> MPKALIVYGSTTGNTEYTAETIARQLANAGYEVD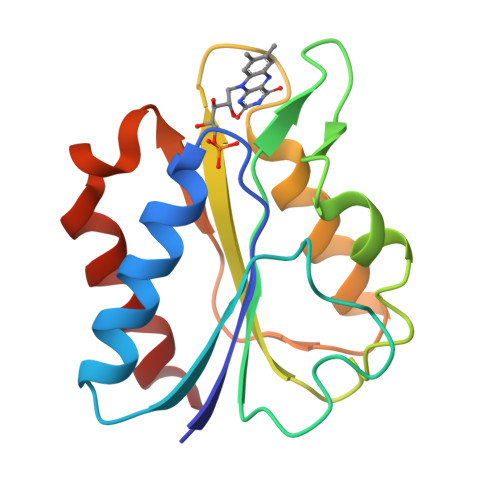SRDAASVEAGGLFEGFDLVLLGCSTWGDDSIELQDDFIPLFDSLEETGAQGRKVACFGCGDSSYEYFCGAVDAIEEKLKNLGAEIVQDGLRIDGDPRAARDDIVGWAHDVRGAI>MGSGLSRVRAVFFDLDNTLIDTAGASRRGMLEVIKLLQSKYHYKEEAEIICDKVQVKLSKECFHPYNTCITDLRTSHWEEAIQETKGGAANRKLAEECYFLWKST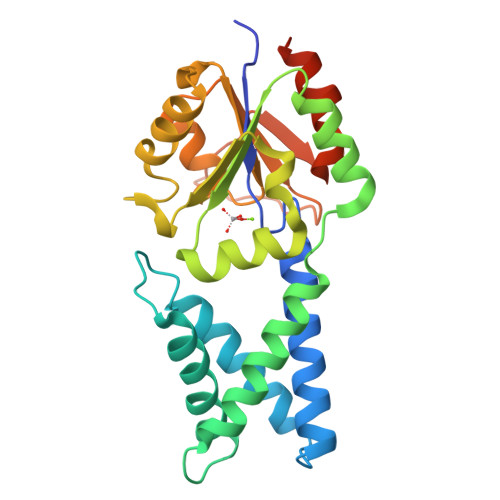RLQHMTLAEDVKAMLTELRKEVRLLLLTNGDRQTQREKIEACACQSYFDAVVVGGEQREEKPAPSIFYYCCNLLGVQPGDCVMVGDTLETDIQGGLNAGLKATVWINKNGIVPLKSSPVPHYMVSSVLELPALLQSIDCKVSMSTEFGLVPR[3x]> MLRFLNQASQGRGAWLLMAFTALALELTALWFQHVMLLKPCVLCIYERVALFGVLGAALIGAIAPKTPLRYVAMVIWLYSAFRGVQLTYEHTMLQLYPSPFATCDFMVRFPE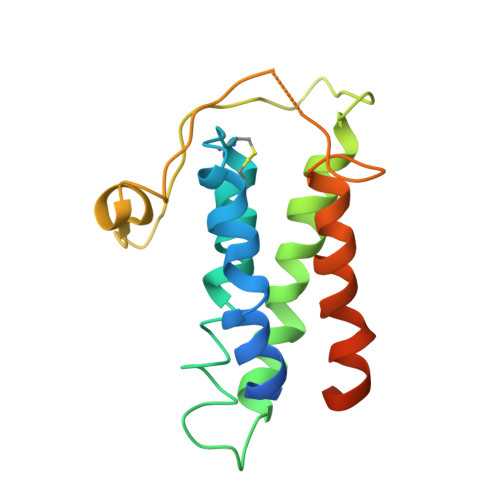WLPLDKWVPQVFVASGDSAERQWDFLGLEMPQWLLGIFIAYLIVAVLVVISQPFKAKKRDLFGR>[2x]SMLERTINLYPLTNYTFGTKEPLYEKDSSVAARFQRMREEFDKIGMRRTVEGVLIVHEHRLPHVLLLQLGTTFFKLPGGELNPGEDEV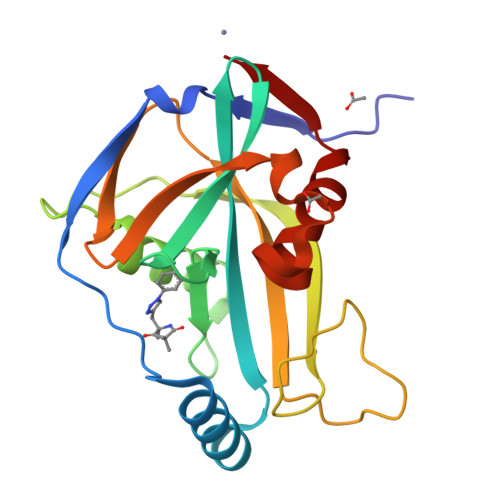EGLKRLMTEILGRQDGVLQDWVIDDCIGNWWRPNFEPPQYPYIPAHITKPKEHKKLFLVQLQEKALFAVPKNYKLVAAPLFELYDNAPGYGPIISSLPQLLSRFNFIYN> MLKKNDIVEVEIVDLTHEGAGVAKVDGLVFFVENALPSEKILMRVLKVNKKIGFGKVEKYLVQSPHRNQDLDLAYLRSGIADLGHLSYPEQLKFKTKQVKDSLYKIAGIADVEVAETLGMEHPVKYRNKAQVPVRRVNGVLETGFFRKNSHNLMPLEDFFIQDPVIDQVVVALRDLLRRFDLKPYDEKEQSGLIRNLVVRRGHYSGQIMVVLVTTRPKVFRVDQLIEQVIKQFPEIVSVMQNINDQNTNAIFGKEWRTLYGQDYITDQMLGNDFQIAGPAFYQVNTEMAEKLYQTAIDFAELK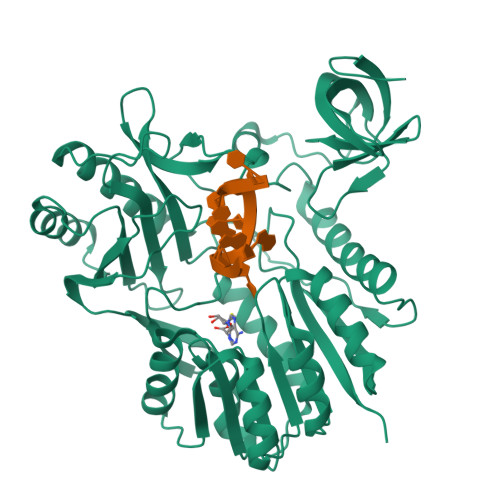KDDVIIDAYSGIGTIGLSVAKHVKEVYGVELIPEAVENSQKNASLNKITNAHYVCDTAENAMKKWLKEGIQPTVILVDPPRKGLTESFIKASAQTGADRIAYISCNVATMARDIKLYQELGYELKKVQPVDLFPQTHHVQTVALLSKLD>YFGKLESKLSVIRNLNDQVLFIDQGNRPLFEDMTDSDCRDNAPRTIFIISMYKDSQPRGMAVTISVKCEKISTLSCENKIISFKEMNPPDNIKDTKSDIIFFQRSVPGHDNKMQFESSSYEGYFLACEKERDLFKLILKKEDELGDRSIMFTVQNED[4x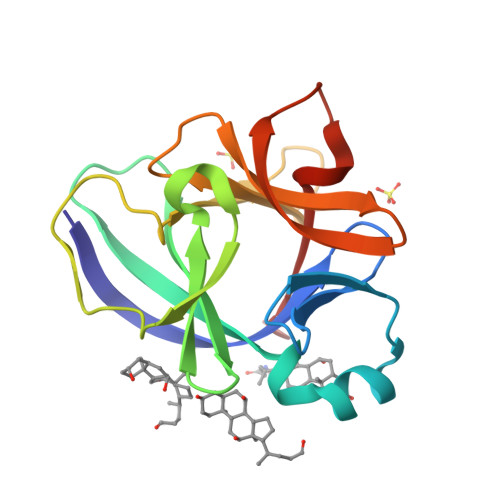]> MSESLSWMQTGDTLALSGELDQDVLLPLWEMREEAVKGITCIDL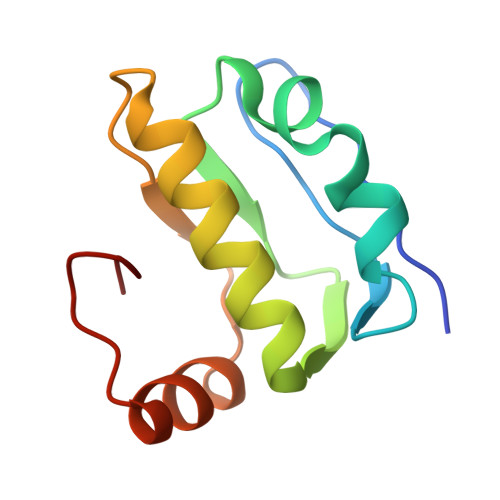SRVSRVDTGGLALLLHLIDLAKKQGNNVTLQGVNDKVYTLAKLYNLPADVLPR>GHMLEMLGTSGVKIHPNGNSNQLGVQLENVKLTSLFKKLDKRCSLASWIKENIKKKECCFYVEDGREGICKCGYPKVQHCDEAIKPEDYMGEQWDKHRHVRETPTDAFGDISFGGLGQKTGKYVRVSSDTSCENLYQLMTEQWKLRSPNLLISVTGGAKNFYIKTHLKDKFRRGLIKVAQTTGAWILTGGTHAGVMKHVGMAVRDYTLSSGSMEGQIVVIGVAPWGVIHNRSTLIHPEGRFPAYYSLDEQGQGRLSCLDINHTHFLLVDDGTQGHYGVEIELRARLEKLISKLSLGNRESGVTIPVVCVVLDGGPGTLNTIYNSMLNHTPCVVLEGSGRLADVIAHVASVPVSKVTMALINRLLKRFFMQEYKNFTELQIIEWTKKIQ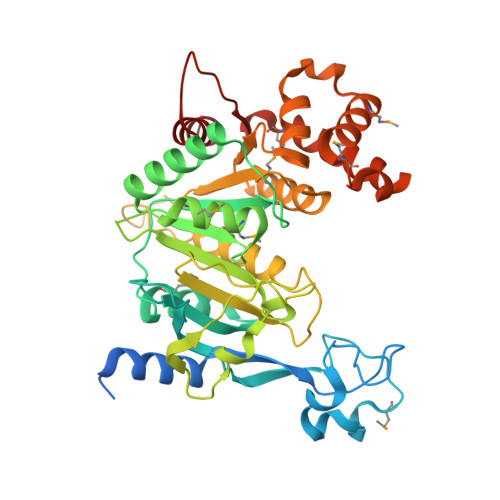DILRMPHLLTVFRIDEDKNYDVDVAILQALLKASRS[2x]5-(5-formylthiophen-2-yl)uridine-5'(2-(acetylamino)-2-deoxy-alpha-D-galactosyl)-diphosphate | C22 H29 N3 O18 P2 S | 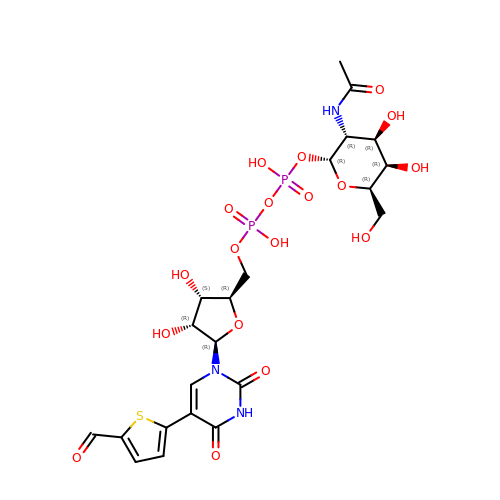PRYRELLFERSIJT-DVUHHYPWSA-N> MPDETNFTIEDIEPRPDALRGLDTQFLQDNTALVQAYRGLDWSDISSLTQMVDVIEQTVVKYGNPNDSIKLALETILWQILRKYPLLFGFWKRFATIEYQLFGLKKSIAVLATSVKWFPTSLELWCDYLNVLCVNNPNETDFIRNNFEIAKDLIGKQFLSHPFWDKFIEFEVGQKNWHNVQRIYEYIIEVPLHQYARFFTSYKKFLNEKNLKTTRNIDIVLRKTQTTVNEIWQFESKIKQPFFNLGQVLNDDLENWSRYLKFVTDPSKSLDKEFVMSVFDRCLIPCLYHENTWMMYIKWLTKKNISDEVVVDIYQKANTFLPLDFKTLRYDFLRFLKRKYRSNNTLFNNIFNETVSRYLKIWPNDILLMTEYLCMLKRHSFKNSLDQSPKEILEKQTSFTKILETSITNYINNQIDAKVHLQTLINDKNLSIVVVELIKTTWLVLKNNMQTRKYFNLYQKNILIKNSVPFWLTYYKFEKSNVNFTKLNKFIRELGVEIYLPTTVMNDILTDYKTFYLTHSNIVTYESSIIDSNTFDPILYPELKMS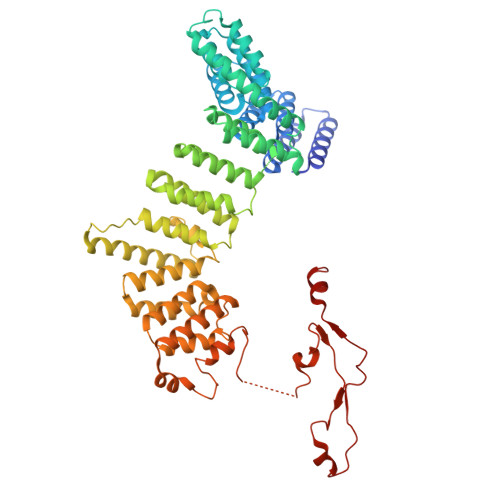NPKYDPVLNTTANVDWHKKTEWKEAGHIGITTERPQISNSIIECNSGTLIQKPISLPNFRNLEKINQVKINDLYTEEFLKEGK>[2x]MEVSPLQPVNENMQVNKIKKNEDAKKRLSVERIYQKKTQLEHILLRPDTYIGSVELVTQQMWVYDEDVGINYREVTFVPGLYKIFDEILVNAADNKQRDPKMSCIRVTIDPENNLISIWNNGKGIPVVEHKVEKMYVPALIFGQLLTSSNYDDDEKKVTGGRNGYGAKLCNIFSTKFTVETASREYKKMFKQTWMDNMGRAGEMELKPFNGEDYTCITFQPDLSKFKMQSLDKDIVALMVRRAYDIAGSTKDVKVFLNGNKLPVKGFRSYVDMYLKDKLDETGNSLKVIHEQVNHRWEVCLTMSEKGFQQISFVNSIATSKGGRHVDYVADQIVTKLVDVVKKKNKGGVAVKAHQVKNHMWIFVNALIENPTFDSQTKENMTLQPKSFGSTCQLSEKFIKAAIGCGIVESILNWVKFKAQVQLNKKCSAVKHNRIKGIPKLDDANDAGGRNSTECTLILTEGDSAKTLAVSGLGVVGRDKYGVFPLRGKILNVREASHKQIMENAEINNIIKIVGLQYKKNYEDEDSLKTLRYGKIMIMTDQDQDGSHIKGLLINFIHHNWPSLLRHRFLEEFITPIVKVSKNKQEMAFYSLPEFEEWKSSTPNHKKWKVKYYKGLGTSTSKEAKEYFADMKRHRIQFKYSGPEDDAAISLAFSKKQIDDRKEWLTNFMEDRRQRKLLGLPEDYLYGQTTTYLTYNDFINKELILFSNSDNERSIPSMVDGLKPGQRKVLFTCFKRNDKREVKVAQLAGSVAEMSSYHHGEMSLMMTIINLAQNFVGSNNLNLLQPIGQFGTRLHGGKDSASPRYIFTMLSSLARLLFPPKDDHTLKFLYDDNQRVEPEWYIPIIPMVLINGAEGIGTGWSCKIPNFDVREIVNNIRRLMDGEEPLPMLPSYKNFKGTIEELAPNQYVISGEVAILNSTTIEISELPVRTWTQTYKEQVLEPMLNGTEKTPPLITDYREYHTDTTVKFVVKMTEEKLAEAERVGLHKVFKLQTSLTCNSMVLFDHVGCLKKYDTVLDILRDFFELRLKYYGLRKEWLLGMLGAESAKLNNQARFILEKIDGKIIIENKPKKELIKVLIQRGYDSDPVKAWKEAQQKVPDEEENEESDNEKETEKSDSVTDSGPTFNYLLDMPLWYLTKEKKDELCRLRNEKEQELDTLKRKSPSDLWKEDLATFIEELEAVEAKEKQDEQVGLPGKGGKAKGKKTQMAEVLPSPRGQRVIPRITIEMKAEAEKKNKKKIKNENTEGSPQEDGVELEGLKQRLEKKQKREPGTKTKKQTTLAFKPIKKGKKRNPWSDSESDRSSDESNFDVPPRETEPRRAATKTKFTMDLDSDEDFSDFDEKTDDEDFVPSDASPPKTKTSPKLSNKELKPQKSVVSDLEADDVKGSVPLSSSPPATHFPDETEITNPVPKKNVTVKKTAAKSQSSTSTTGAKKRAAPKGTKRDPALNSGVSQKPDPAKTKNRRKRKPSTSDDSDSNFEKIVSKAVTSKKSKGESDDFHMDFDSAVAPRAKSVRAKKPIKYLEESDEDDLF

The human type IIA topoisomerases (Top2) are essential enzymes that regulate DNA topology and chromosome organization. The passage of the T-segment requires ATP hydrolysis and is thought to occur along with the opening and closing of several dimeric interfaces constituting molecular gates. In this work, we determined the cryo-EM structure of the full-length human Topo IIα isoform bound to DNA in different conformations trapped by the anti-cancer drug etoposide.

State 1 was solved at 3.6 Å using 60,601 particles and State 2 was solved at 4.1 Å using 39,368 particles. The well-resolved EM density of the 3.6 Å map in State 1 allowed us to fit, build and refine the atomic model of the hTopo IIα DNA-binding/cleavage domain in complex with DNA and etoposide27. Strikingly, we were also able to identify EM density for the etoposide molecule, intercalating in the DNA duplex between positions −1 and +1, with similar protein and DNA contacts as previously reported in crystallographic structures. In State 1, the TOPRIM and Tower domains are positioned upward and tightly bound to the G-segment which is highly bent. This state corresponds to a closed cleavage complex as observed in the structure of the DNA-bound hTopo IIα DNA-binding/cleavage domain crystallized without etoposide, with the exception of the C-gate being closed in our structure. However, analysis of the 3.6 Å EM map of the DNA binding/cleavage domain revealed an additional EM density that could be attributed to the beginning of the CTD domain (residues 1192–1215). This region of the CTD begins at the end of the terminal coiled-coil alpha helix of the DNA binding/cleavage domain on residue 1192, stretches along the Tower domain and extends under the G-segment major groove pointing in an orthogonal direction from the DNA gate. In addition, the 3.6 Å structure of the DNA-binding/cleavage domain reveals a part of the CTD domain which was not previously observed and is positioned nearby the G-segment inflection points on each side of the enzyme. The particular localization of the CTD linker may structurally favor the curvature of the G-segment, stimulating DNA cleavage and favoring strand passage. The portion of the CTD ranging from residue 1192 to residue 1217 is in close vicinity of the G-segment and seems to act as a positive regulator of the strand passage process, which appears to stimulate the relaxation activity and stabilize the cleavage complex in presence of etoposide.>GPLGSEADPRLIESLSQMLSMGFSDEGGWLTRLLQTKNYDIGAALDTIQYSKH[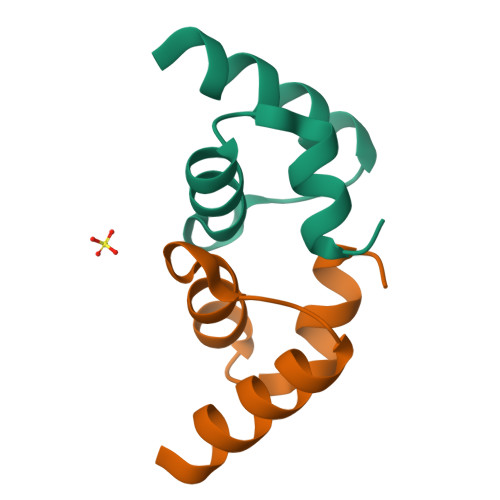2x]>GIDPFTNTKWDYKNKENGPHRWDKLHKDFEVCKSGKSQSPINIEHYYHTQDKADLQFKYAASKPKAVFFTHHTLKASFEPTNHINYRGHDYVLDNVHFHAP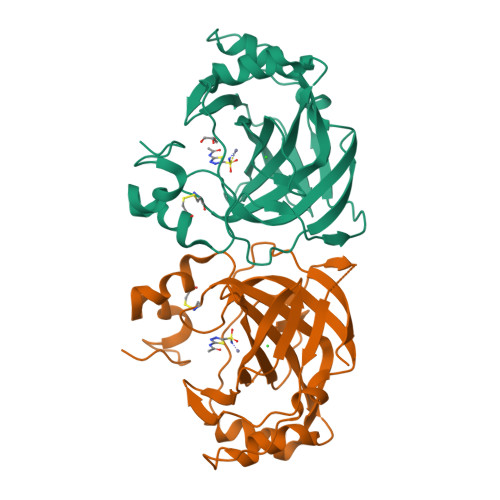MEFLINNKTRPLSAHFVHKDAKGRLLVLAIGFEEGKENPNLDPILEGIQKKQNFKEVALDAFLPKSINYYHFNGSLTAPPCTEGVAWFVIEEPLEVSAKQLAEIKKRMKNSPNQRPVQPDYNTVIIKSSAETR[8x]>MSKSWGKFIEEEEAEMASRRNLMIVDGTNLGFRFKHNNSKKPFASSYVSTIQSLAKSYSARTTIVLGDKGKSVFRLEHLPEYAGNRDEKYAQRTEEEKALDEQFFEYLKDAFELCKTTFPTFTIRGVEADDMAAYIVKLIGHLYDHVWLISTDGDWDTLLTDKVSRFSFTTRREYHLRDM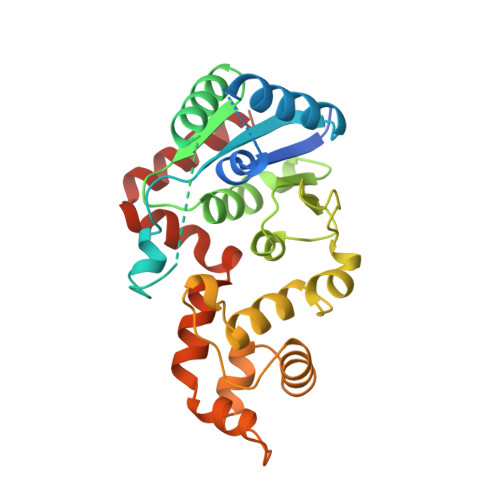YEHHNVDDVEQFISLKAIMGDLGDNIRGVEGIGAKRGYNIIREFGNVLDIIDQLPLPGKQKYIQNLNASEELLFRNLILVDLPTYCVDAIAAVGQDVLDKFTKDILEIAEQ[2x]>GSAAAQDMVSPPPPIADEPLTVNTGIYLIESYSLDDCAETFKVNAFLSLSWKDRRLAFDPVRSGVRVKTYEPEAIWIPEIRFVNVENARDADVVDISVSPDGTVQYLERFSARVLSPLDFRRYPFDSQTLHIYLIVRSVDTRNIVLAVDLEKVGKNDDVFLTGWDIESFTAVVKPANFALEDRLESKLDYQLRISRQYFSYIPNIILPMLFILFISWTAFWSTSYEANVTLVVSTLIAHIAFNILVETCLPKTPYMTYTGAIIFMIYLFYFVAV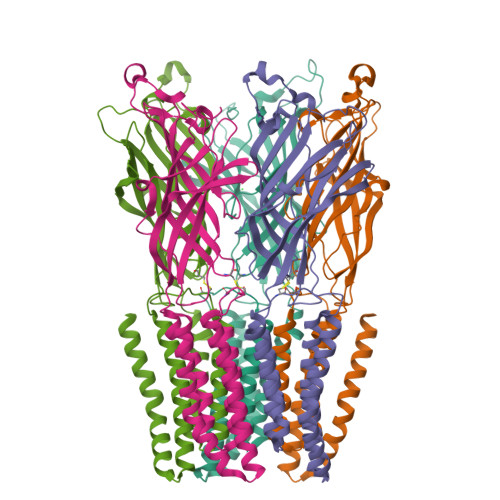IEVTVQHYLKVESQPARAASITRASRIAFPVVFLLANIILAFLFFGF[5x]> MEIVEYPDPILRAKNKRIDIFDENLKNLVDAMFDVMYKTDQIGLSAPQVGLNVQLMVFNPAGEPGEGKEIVLVNPKIKKYSDKLVPFDEGCLSFPGIYAEVVRPQSVKIDARDITGERFSISLSRLPARIFQHEYDHLEGVLFFDRMTDQVLDSIREE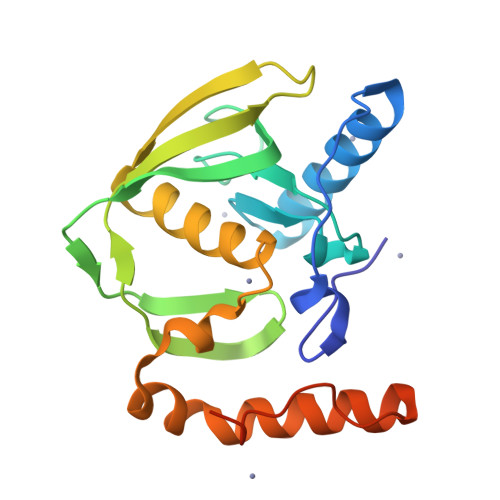LEALEKKYEEKTGLPSPERVEARQKRKAGVGFGKR>MARKTKVTPDDNSIIDLGPRVQSLMEQLATTKLEEGVKNLDMGSVYEITTVMVLGNSILGFHKGDLVKMVRPSVSARDLIGVGYATASAAVVRQRLIEHKIEAGAELIISGTAGGKTVLTNHYAAQMCAKGLKVAVVSMAEAERPLYGSVLHVFAALHLAAVSDVDVLYVDSLRSVYNELGGNLKKGGVSRQVDGMLTALDQYARAVNMRVVFTLNPSDDENVDAAVRSVFKTASASMHTARRIKSFAVNGTAFTAETEIHLRADRSNSANRVSGDLVSRGVSNANAIGAVFNQFLLSGQDGSAFLGPNIPESNYIEGVDK[12x]

The lipid-enveloped bacteriophages of the Cystoviridae family infect Gram-negative bacteria, mainly plant-pathogenic Pseudomonas species and share similarities with the members of the Reoviridae family, including bluetongue virus and rotavirus. Their genome of ∼14 kb consists of three dsRNA segments small (S), medium (M) and large (L), which are sequentially encapsidated as ssRNA precursors into the icosahedrally symmetric procapsid by the packaging NTPase P4 (15–23). P4 is a protein of ∼35 kDa, which can assemble into a hexameric ring. NTP-binding sites are located on the external perimeter of the ring at the interfaces between adjacent subunits, whereas the nucleic acid binding sites are found in the central channel. P4 proteins are the only known RNA-specific helicases belonging to helicase Superfamily 4 (SF4).

The ɸ8 P4 N-terminal domain is composed of two helices separated by a four-stranded antiparallel β-sheet. In P4 ɸ8, the strand following the arginine fingers motifs does not extend as far as the ATP-binding site but instead climbs back along the side of the hexamer (partially disordered) to re-emerge into as C-terminal helix at the top of the hexamer, followed by a loop that dives into the central channel restricting its diameter by more than half (see later in the text for more discussion on the C-terminal domain). However, in ɸ8 P4, these residues are displaced >8 Å from that position and therefore cannot contribute to catalysis. This suggests that in ɸ8 P4, extensive conformational changes occur as a consequence of nucleotide and/or oligonucleotide binding, which render the enzyme competent for catalysis. Although the L2 loop of ɸ8 P4 contains hydrophilic residues (DDENVD), it does not project a lysine side chain towards the central channel. Nevertheless, the L1 loop contains a motif (LKK) that has been shown to be crucial for RNA binding. The first lysine of this motif (K185) is found in the equivalent position to K241 of ɸ12 P4 and is also seen interacting with D220 of loop L2. We therefore postulate that K185 (loop L1) in ɸ8 P4 plays the same role in RNA binding as K241 (loop L2) in ɸ12 P4, and that the coupling of the movement of the L1 and L2 loops to ATP hydrolysis via motion of helix 6, as proposed for ɸ12, may be a general feature of all P4 molecules. As the C-terminal domain is (i) necessary for ATP hydrolysis (data not shown), (ii) restricts the diameter of the central channel and (iii) blocks the interface through which RNA is thought to be loaded, we postulate that the C-terminal region needs to be displaced by RNA for ring opening and subsequent ATP hydrolysis to occur. Thus, it appears that ɸ8 P4 has developed a specific mechanism to regulate ATPase activity and couple it with ssRNA binding such that RNA displaces the C-terminal domain, to allow ATP hydrolysis to occur.> IGIPFPDHSSDILSGLNEQRTQGLLCDVVILVEGREFPTHRSVLAACSQYFKKLF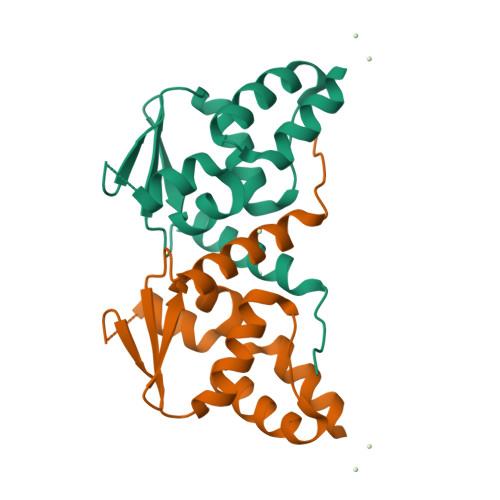TSGAVVDQQNVYEIDFVSAEALTALMDFAYTATLTVSTANVGDILSAARLLEIPAVSHVCADLLD> IAGGEAITTGGSRCSLGFNVSVNGVAHALTAGHCTNISASWSIGTRTGTSFP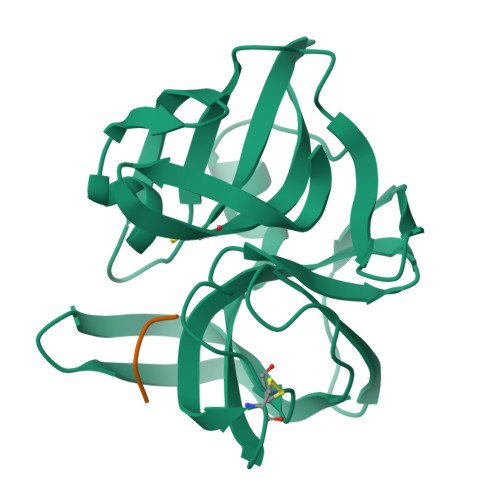NNDYGIIRHSNPAAADGRVYLYNGSYQDITTAGNAFVGQAVQRSGSTTGLRSGSVTGLNATVNYGSSGIVYGMIQTNVCAQPGDSGGSLFAGSTALGLTSGGSGNCRTGGTTFYQPVTEALSAYGATVL;> XPAPY>[2x]MDTGEASYYGSRHAGLRTASGERYNPNAMTAAHRTLPFGAR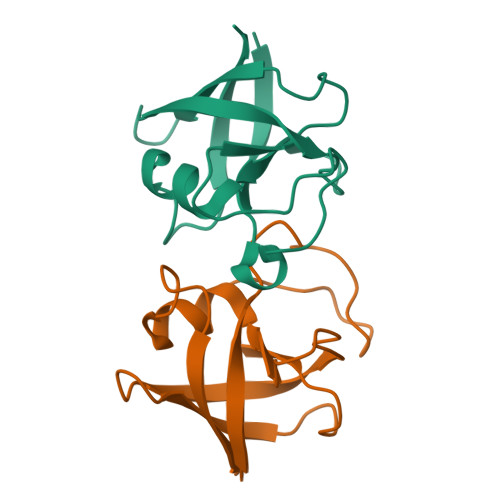VRVTNLDNRRSVVVRINDRGPFRRGRIIDVSRKAAEGLGMIRSGVAPVRIESLD>[8x]MTKRKLAYIWSLRNAAADKAGQYVPYKGEQRYMKSVLESLVEALNQTALGDAYELVGVIYDDDAELPRDQGKIKDYGFAYRPGQQWFYPADLQVQGKTLNDLLLSVPSTYRRYPRGTPEHVAGKSDFERRLHDTLVELGADV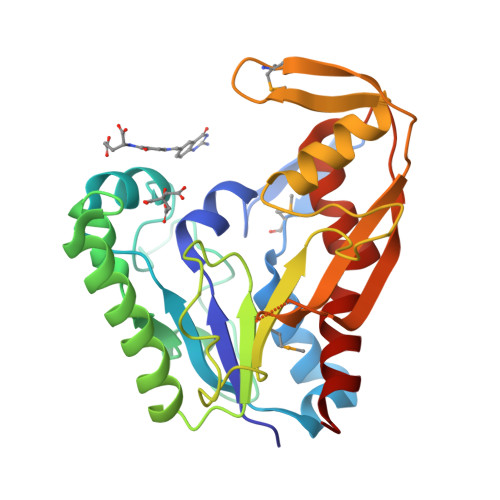VVLDGLLVILDELVRPGAPFARRIMNIHPGVTREDSPYERRGAYATLDALYGARGEKVVDWATMEKVAVEPLYWTGASFHYVDNGIDSGEVFHDVLKTEISPDDTILELRWNNFNNSLFPALHEGLALLAEKL> GSKQQTSALIHNIFDSHFAAIQIHHDSNSKSEVIRDFYTDRDTDVLNFFFLSIDQSDPSHTPEFRFLTDHKGIIWDDGNAHFYGVNDLILDSLANRVSFSNNWYYINVMTSIGSRHMLVRRVPILDPSTGEVLGFSFNAVVLDNNFALMEKLKSESNVDNVVLVANSVPLANSLIGDEPYNVADVLQRKSSDKR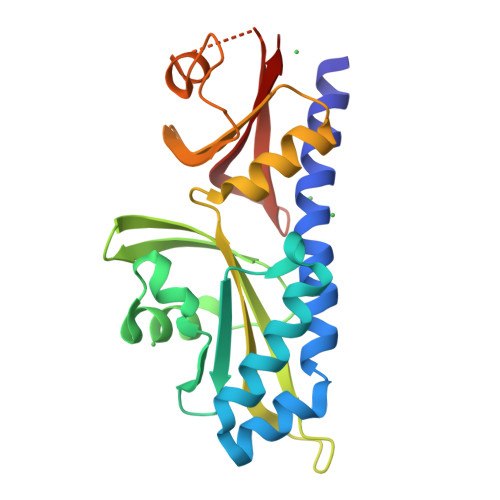LDKLLVIETPIVVNAVTTELCLLTVQD> MTRLFMLVCLGIVCQGTTGNILRGESLNKSLPILHEWKFFDYDFGSDERRQDAILSGEYDYKNNYPSDIDQWHDKIFVTMLRYN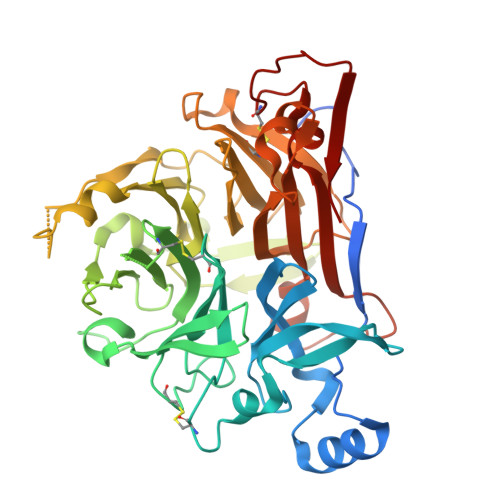GVPSSLNVISKKVGDGGPLLQPYPDWSFAKYDDCSGIVSASKLAIDKCDRLWVLDSGLVNNTQPMCSPKLLTFDLTTSQLLKQVEIPHDVAVNATTGKGRLSSLAVQSLDCNTNSDTMVYIADEKGEGLIVYHNSDDSFHRLTSNTFDYDPKFTKMTIDGESYTAQDGISGMALSPMTNNLYYSPVASTSLYYVNTEQFRTSDYQQNDIHYEGVQNILDTQSSAKVVSKSGVLFFGLVGDSALGCWNEHRTLERHNIRTVAQSDETLQMIASMKIKEALPHVPIFDRYINREYILVLSNKMQKMVNNDFNFDDVNFRIMNANVNELILNTRCENPDNDRTPFKISIHL> DCPSGWSSYEGHCYKPFKLYKTWDDAERFCTEQAKGGHLVSIE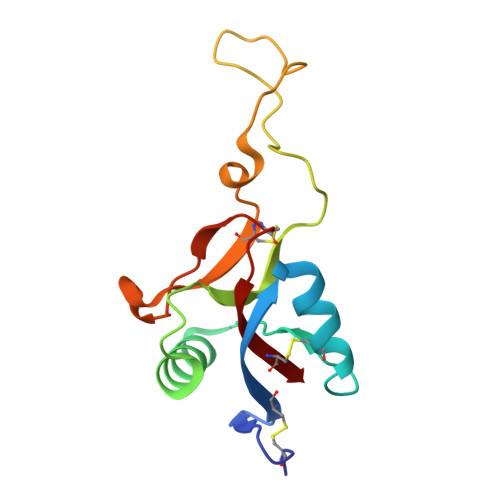SAGEADFVAQLVTENIQNTKSYVWIGLRVQGKEKQCSSEWSDGSSVSYENWIEAESKTCLGLEKETGFRKWVNIYCGQQNPFVCEA>[2x]MRDHRKIGKQLDLYHMQEEAPGMVFWHNDGWTIFRELEVFVRSKLKEYQYQEVKGPFMMDRVLWEKTGHWDNYKDAMFTTSSENREYCIKPMNCPGHVQIFNQGLKSYRDLPLRMAEFGSCHRNEPSGSLHGLMRVRGF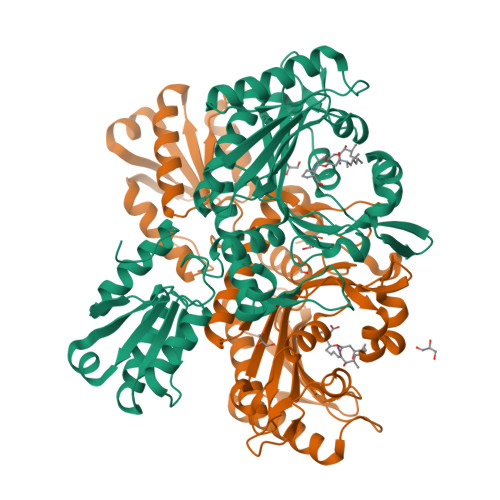TQDDAHIFCTEEQIRDEVNGCIRLVYDMYSTFGFEKIVVKLSTRPEKRIGSDEMWDRAEADLAVALEENNIPFEYQLGEGAFYGPKIEFTLYDCLDRAWQCGTVQLDFSLPSRLSASYVGEDNERKVPVMIHRAILGSMERFIGILTEEFAGFFPTWLAPVQVVIMNITDSQSEYVNELTQKLSNAGIRVKADLRNEKIGFKIREHTLRRVPYMLVCGDKEVESGKVAVRTRRGKDLGSMDVNEVIEKLQQEIRSRSLKQLEELEHHHHHH>[3x]MNHKVHHHHHHIEGRHMAVVKEVLEIAEKIKNMEIRGAGKIARSAAYALQLQAEKSKATNVDEFWKEMKQAAKILFETRPTAVSLPNALRYVMHRGKIAYSSGADLEQLRFVIINAAKEFIHNSEKALERIGEFGAKRIEDGDVIMTHSHSKAAISVMKTAWEQGKDIKVIVTETRPKWQGKITAKELASYGIPVIYVVDSAARHYMKMTD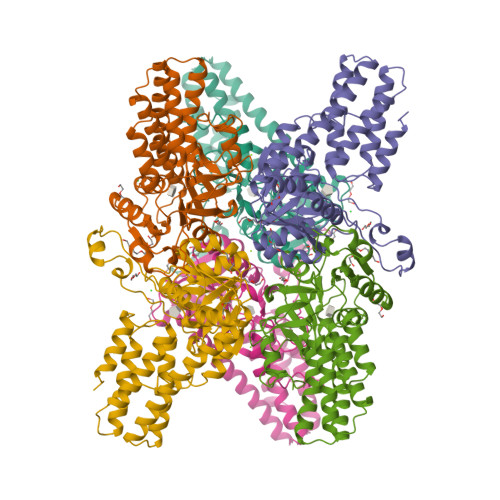KVVMGADSITVNGAVINKIGTALIALTAKEHRVWTMIAAETYKFHPETMLGQLVEIEMRDPTEVIPEDELKTWPKNIEVWNPAFDVTPPEYVDVIITERGIIPPYAAIDILREEFGWALKYTEPWED> MRGSHHHHHHGRSLNPLSTPQFDSTDETPASYNLAVRRAAPAVVNVYNRGLNTNSHNQLEIRTLGSGVIMDQRGYIITNKHVINDADQIIVALQDGRVFEAL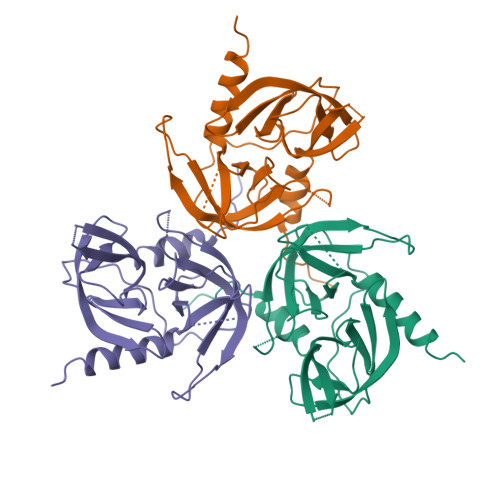LVGSDSLTDLAVLKINATGGLPTIPINARRVPHIGDVVLAIGNPYNLGQTITQGIISATGRIGLNPTGRQNFLATDASINHGNSGGALVNSLGELMGINTLSFDKSNDGETPEGIGFAIPFQLATKIMDKLIRDGRVIR>[72x]MGLFDRIKRVVSSNLNDLVNKAEDPEKMLEQAILEMQEDLVQLRQGVAQAIAAQKRSEKQYNDAQNEINKWQRNAQLALQKGDENLARQALERKKTYTDTSAALKASLDTQSTQVETLKRNLIQLESKISEAKTKKEMLKARITTAKAQEQLQGMVRGMNTSSAMSAFERMEEKVLMQESRAQALGELAGADLETQFAQLEGGS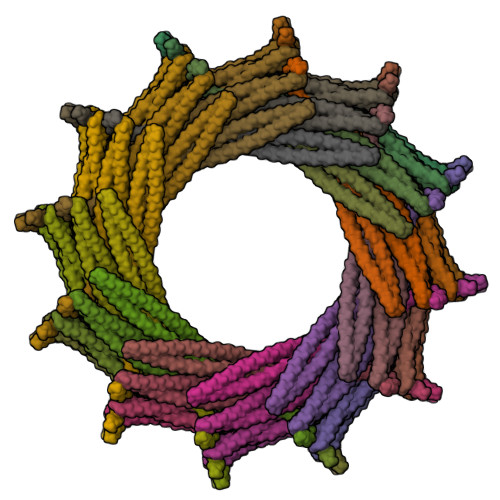DVDDELAALKAQMLPPATPVTQAQLPPQQETTPAKSNEVVDAELDSLRKQLDQL> GPGSMGLRWLQAALVCTSLAAGLSAAAPARAQGAAPVKIGFVVKQPDDPWFQDEWRFAEQAAKDKHFTLVKIAAPSGEKVSTALDSLAAQKAQGVIICAPDVKLGPGIAAKAKRYGMKLMSVDDQLVDGRGAPLADVPHMGISAYRIGRQVGDAIA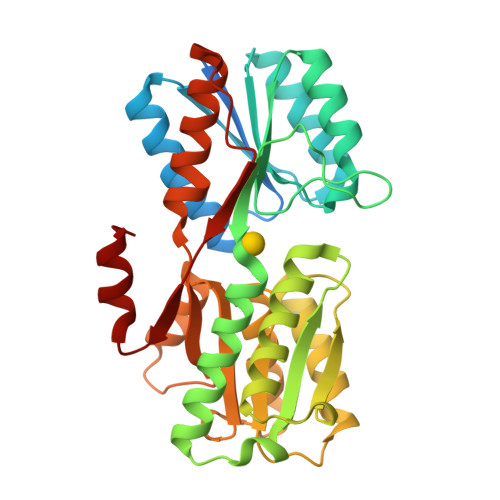AEAKRRGWNPAEVGVLRLAYDQLPTARERTTGAVDALKAAGFAAANVVDAPEMTADTEGAFNAANIAFTKHRNFRHWVAFGSNDDTTVGAVRAGEGRGIGTDDMIAVGINGSQVALNEFAKPKPTGFFGSILLNPRLHGYDTSVNMYDWITQNRTPPPLVLTSGTLITRANEKTARAQLGL>DYKDDDDKLHSQANLMRLKSDLFNRSPMYPGPTKDDPLTVTLGFTLQDIVKADSSTNEVDLVYYEQQRWKLNSLMWDPNEYGNITDFRTSAADIWTPDITAYSSTRPVQVLSPQIAVVTHDGSVMFIPAQRLSFMCDPTGVDSEEGATCAVKFGSWVYSGFEIDLKTDTDQVDLSSYYASSKYEILSATQTRQVQHYSCCPEPYIDVNLVVKFRER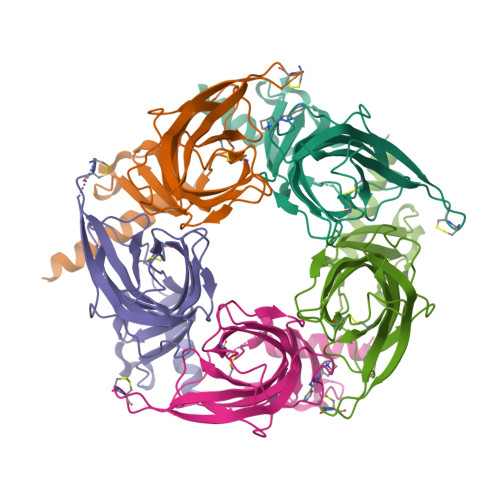[5x]> QRVIPVYQVNNLEEICQLIIQAFEAGVDFQESADSFLLMLCLHHAYQGDYKLFLESGAVKYLEGHGFRFEVKKRDGVKRLEELLPAVSSGKNIKRTLAAMPEEETTEANAGQFLSFASLFLPKLVVGEKACLEKVQRQIQVHAEQGLIQYPTAWQSVGHMMVIFRLMRTNFLIKFLL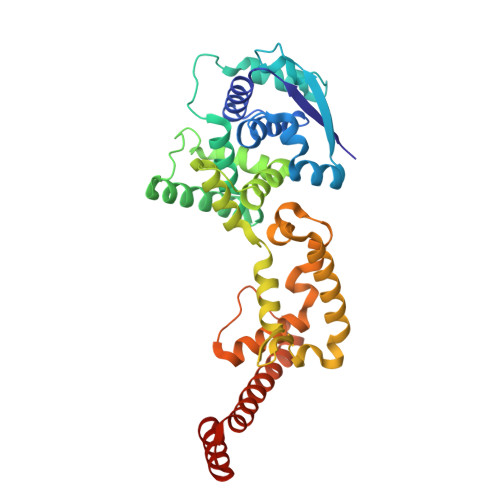IHQGMHMVAGHDANDAVISNSVAQARFSGLLIVKTVLDHILQKTERGVRLHPLARTAKVKNEVNSFKAALSSLAKHGEYAPFARLLNLSGVNNLEHGLFPQLSAIALGVATAHGSTLAGVNVGEQYQQLREAATEAEKQLQQYAESRELDHLGLDDQEKKILMNFHQKKNE> MTTSVFVSGATGYLAQQIIALVLSKGYKVVGSVRSEEKGANLKKLYGDDFSYEVVKVLEQKGAFDEALKKHPEVTIFLHTASPVTFEVEDTEKEILIPAINGTKYVLQSIKDVAPQITRVVYTSSVVAMSVPEELGSPDVVLSEASWSSLSYEQSKTHGVLAYFGSKQFAERAAWEFVEQEKPNFALSTVNPVYIFGPQAKDEEVKGTLNLSAEMVNSVLKLNKDDDVPATTGTFIDVRDVAKAHLAAFEKDEAKGERLLLSNTRFNGQTLLDVVRKNFPQL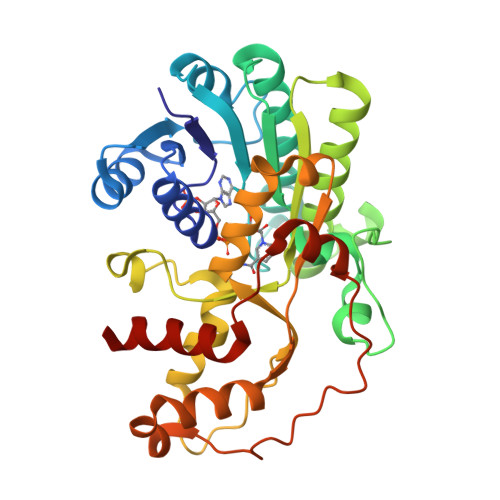ADKLPVGKPHSDDFSAFKEWNDKKTKKILGFEYFDFETSVVDSIKQVLKVQG>[2x]MHTDTTRENPQA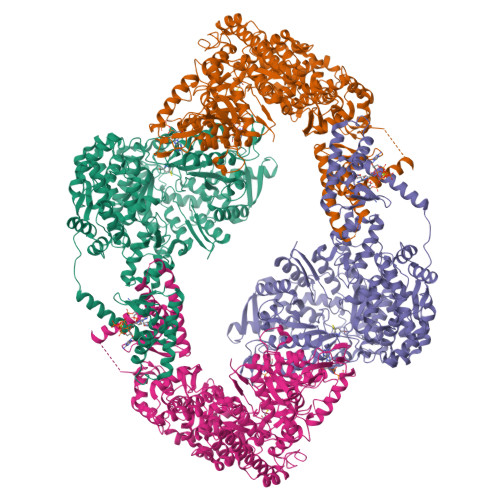SAPQAADSSQDLAATAPGQLRVIKRNGTVVPYTDDKITVAITKAFLAVEGGTAAASSRIHDTVRRLTEQVTATFKRRMPSGGTIHIEEIQDQVELALMRAGEQKVARDYVIYREARAAERKNAGAASDVAQPHPSIRITRADGSLSPLDMGRLNTIISEACEGLAEVDGALIERETLKNLYDGVAEKDVNTALVMTARTLVEREPNYSYVTARLLMDTLRAEALGFLGVAESATHHEMAELYAKALPAYIEKGAEFELVDAKLKEFDLEKLGKAIDHERDQQFTYLGLQTLYDRYFIHKDGIRFELPQIFFMRVAMGLAIEEKDREARAIEFYNLLSSFDYMSSTPTLFNAGTLRPQLSSCYLTTVPDDLSGIYGAIHDNAMLSKFAGGLGNDWTPVRALGSYIKGTNGKSQGVVPFLKVVNDTAVAVNQGGKRKGAVCAYLETWHLDIEEFLELRKNTGDDRRRTHDMNTANWIPDLFMKRVFDDGSWTLFSPSDVPDLHDLYGKAFEERYEYYEALASYGKLKLHKVVQAKDLWRKMLSMLFETGHPWLTFKDPCNLRSPQQHVGVVHSSNLCTEITLNTNKDEIAVCNLGSINLVNHIVDGKLDTAKLEKTVKTAVRMLDNVIDINYYSVPQAQNSNFKHRPVGLGIMGFQDALYLQHIPYGSDAAIAFADQSMEAISYYAIQASCDLADERGAYQTFQGSLWSQGILPIDSEKKLIEERGAKYIEVDLSETLDWAPLRERVQKGIRNSNIMAIAPTATIANITGVSQSIEPTYQNLYVKSNLSGEFTVINPYLVRDLKARGLWDPVMVNDLKYYDGSVQQIERIPQDLKDLYATAFEVETRWIVEAASRRQKWIDQAQSLNLYIAGASGKKLDVTYRMAWFRGLKTTYYLRALAATSTEKSTINTGKLNAVSAGGNDGLQAAPAAEPKPAPVPQACSIDNPDCEACQ>GQDMVSPPPPIADEPLTVNTGIYLIECYSLDDKAATFKVNAFLSLSWKDRRLAFDPVRSGVRVKTYEPEAIWIPEIRFVNVENARDADVVDISVSPDGTVQYLERFSARVLSPLDFRRYPFDSQTLHIYLIVRSVDTRNIVLAVDLEKVGKNDDVFLTGWDIESFTAVVKPANFALEDRLESKLDYQLRISRQYFSYIPNIILPMLFILFISWTAFWSTSYEANVTLVVSTLIAHIAFNILVETNLPKTPYMTYTGAIIFMIYLFYFVAVIEVTVQHYLKVESQPARAASITRASRIAFPVVFLLANIILAFLFFGF[5x]

At present, the best structurally characterized pLGIC is the G. violaceus ligand-gated ion channel (GLIC), of prokaryotic origin. Each subunit consists of an extracellular domain (ECD), predominantly in a β-sandwich fold, and a transmembrane domain (TMD) composed of four helices, labeled M1–M4. However, the GLIC is a pH-gated channel, activated by lowering the pH, with a maximal activation at pH 4 and a pH50 around 5. We instead found that proton activation is a complex multiple loci mechanism, with the key contribution stemming from the coupling interface between the extracellular and transmembrane domain, with E35 acting as a key proton-sensing residue.

Finally, mutation of E35 produced the strongest effect; therefore, a more extensive study of this position was performed. The mutations E35Q, E35A, and E35M (the GlyR-position equivalent) display a significant increase in pH50, whereas E35K shows a weaker nonsignificant effect, and E35H appears to show the inverse phenotype with a marked decrease in pH50. Altogether, these data show that the loss of charge at the E35 position is important to the gain-of-function effect found. Mutants of E35 are unique in strongly increasing the proton sensitivity. Neutralization of the E35 side chain by mutation to A, Q, or M produce a similar increase in proton sensitivity, whereas the mutation of E35K exhibits the same behavior with half the increase. Interestingly, the structures of the Wt GLIC, E35Q, and E35A at pH 4 show that the side chain of residue 35 is located in a hydrophobic environment bordered by the side chains of P113, L114, F116, F156, T158, and P247. There are no significant differences, measured as 5-fold over Wt, seen in the backbone Cα residues of any of the resolved structures, with the exception of E35A and E82Q. Interestingly, E35A also produces the greatest structural deviations around Y28 along with neighboring residues. Altogether, the data support that E35 is a bona fide proton sensor, whose charged form stabilizes the resting conformation, whereupon protonation favors the active state. The functional proton gating of E35Q and E35A mutants additionally suggests that if E35 is a bona fide proton sensor, it can’t be the only one in the GLIC.> MEGNKLEEQDSSPPQSTPGLMKGNKREEQGLGPEPAAPQQPTAEEEALIEFHRSYRELFEFFCNNTTIHGAIRLVCSQHNRMKTAFWAVLWLCTFGMMYWQFGLLFGEYFSYPVSLNINLNSDKLVFPAVTICTLNPYRYPEIKEELEELDRITEQTLFDLYKYSSFTTLVAGSRSRRDLRGTLPHPLQRLRVPPPPHGARRARSVASSLRDNNPQVDWKDWKIGFQLCNQNKSDCFYQTYSSGVDAVREWYRFHYINILSRLPETLPSLEEDTLGNFIFACRFNQVSCNQANYSHFHHPMYGNCYTFNDKNNSNLWMSSMPGINNGLSLMLRAEQNDFIPLLSTVTGARVMVHGQDEPAFMDDGGFNLRPGVETSISMRKETLDRLGGDYGDCTKNGSDVPVENLYPSKY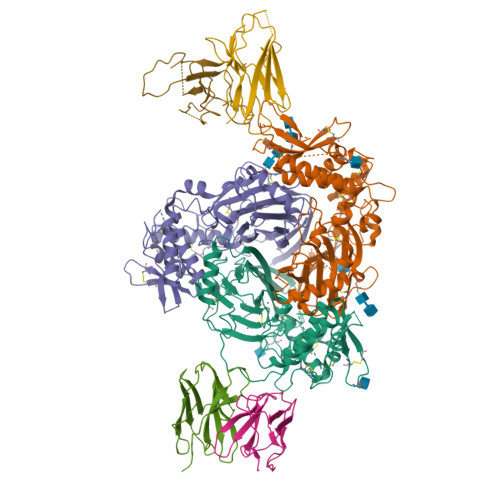TQQVCIHSCFQESMIKECGCAYIFYPRPQNVEYCDYRKHSSWGYCYYKLQVDFSSDHLGCFTKCRKPCSVTSYQLSAGYSRWPSVTSQEWVFQMLSRQNNYTVNNKRNGVAKVNIFFKELNYKTNSESPSVTMVTLLSNLGSQWSLWFGSSVLSVVEMAELVFDLLVIMFLMLLRRFRSRYWSPGRGGRGAQEVASTLASSPPSHFCPHPMSLSLSQPGPAPSPALTAPPPAYATLGPRPSPGGSAGASSSTCPLGGP;> MHVKKYLLKGLHRLQKGPGYTYKELLVWYCDNTNTHGPKRIICEGPKKKAMWFLLTLLFAALVCWQWGIFIRTYLSWEVSVSLSVGFKTMDFPAVTICNASPFKYSKIKHLLKDLDELMEAVLERILAPELSHANATRNLNFSIWNHTPLVLIDERNPHHPMVLDLFGDNHNGLTSSSASEKICNAHGCKMAMRLCSLNRTQCTFRNFTSATQALTEWYILQATNIFAQVPQQELVEMSYPGEQMILACLFGAEPCNYRNFTSIFYPHYGNCYIFNWGMTEKALPSANPGTEFGLKLILDIGQEDYVPFLASTAGVRLMLHEQRSYPFIRDEGIYAMSGTETSIGVLVDKLQRMGEPYSPCTVNGSEVPVQNFYSDYNTTYSIQACLRSCFQDHMIRNCNCGHYLYPLPRGEKYCNNRDFPDWAHCYSDLQMSVAQRETCIGMCKESCNDTQYKMTISMADWPSEASEDWIFHVLSQERDQSTNITLSRKGIVKLNIYFQEFNYRTIEESAANNIVWLLSNLGGQFGFWMGGSVLCLIEFGEIIIDFVWITIIKLVALAKSLRQRRAQASYAGPPPTVAELVEAHTNFGFQPDTAPRSPNTGPYPSEQALPIPGTPPPNYDSLRLQPLDVIESDSEGDAI;> MAPGEKIKAKIKKNLPVTGPQAPTIKELMRWYCLNTNTHGCRRIVVSRGRLRRLLWIGFTLTAVALILWQCALLVFSFYTVSVSIKVHFRKLDFPAVTICNINPYKYSTVRHLLADLEQETREALKSLYGFPESRKRREAESWNSVSEGKQPRFSHRIPLLIFDQDEKGKARDFFTGRKRKVGGSIIHKASNVMHIESKQVVGFQLCSNDTSDCATYTFSSGINAIQEWYKLHYMNIMAQVPLEKKINMSYSAEELLVTCFFDGVSCDARNFTLFHHPMHGNCYTFNNRENETILSTSMGGSEYGLQVILYINEEEYNPFLVSSTGAKVIIHRQDEYPFVEDVGTEIETAMVTSIGMHLTESFKLSEPYSQCTEDGSDVPIRNIYNAAYSLQICLHSCFQTKMVEKCGCAQYSQPLPPAANYCNYQQHPNWMYCYYQLHRAFVQEELGCQSVCKEACSFKEWTLTTSLAQWPSVVSEKWLLPVLTWDQGRQVNKKLNKTDLAKLLIFYKDLNQRSIMESPANSIEMLLSNFGGQLGLWMSCSVVCVIEIIEVFFIDFFSIIARRQWQKAKEWWAWKQAPPCPEAPRSPQGQDNPALDIDDDLPTFNSALHLPPALGTQVPGTPPPKYNTLRLERAFSNQLTDTQMLDEL> MKRDHHQFQGRLSNHGTSSSSSSISKDKMMMVKKEEDGGGNMDDELLAVLGYKVRSSEMAEVALKLEQLETMMSNVQEDGLSHLATDTVHYNPSELYSWLDNMLSELNPPPLPASSNGLDPVLPSPEICGFPASDYDLKVIPGNAIYQFPAIDSSSSSNNQNQQLQSCSSPDSMVTSTSTGTQIGGVIGTTVTTTTTTTTAAGESTRSVILVDSQENGVRLVHALMACAEAIQQNNLTLAEALVKQIGCLAVSQAGAMRKVATYFAEALARRIYRLSPPQNQIDHCLSDTLQMHFYETCPYLKFAHFTANQAILEAFEGKKRVHVIDFSMNQGLQWPALMQALALREGGPPTFRLTGIGPPAPDNSDHLHEVGCKLAQLAEAIHVEFEYRGFVANSLAD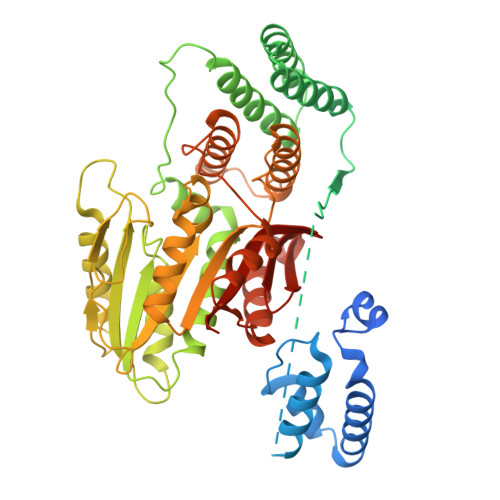LDASMLELRPSDTEAVAVNSVFELHKLLGRPGGIEKVLGVVKQIKPVIFTVVEQESNHNGPVFLDRFTESLHYYSTLFDSLEGVPNSQDKVMSEVYLGKQICNLVACEGPDRVERHETLSQWGNRFGSSGLAPAHLGSNAFKQASMLLSVFNSGQGYRVEESNGCLMLGWHTRPLITTSAWKLSTAAYGGWSHPQFER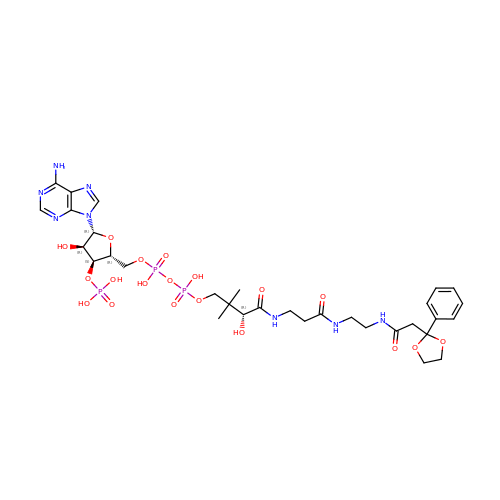[(2R,3S,4R,5R)-5-(6-amino-9H-purin-9-yl)-4-hydroxy-3-(phosphonooxy)oxolan-2-yl]methyl (3R)-3-hydroxy-2,2-dimethyl-4-oxo-4-{[3-oxo-3-({2-[2-(2-phenyl-1,3-dioxolan-2-yl)acetamido]ethyl}amino)propyl]amino}butyl dihydrogen diphosphate | C32 H47 N8 O19 P3 | ZFQRYYBRRRMTLD-HSJNEKGZSA-N>[3x]MAFSARFPLWLLLGVVLLASVSASFAHSGHSGGEAEDESEESRAQNNPYLFRSNKFLTLFKNQHGSLRLLQRFNEDTEKLENLRDYRVLEYCSKPNTLLLPHHSDSDLLVLVLEGQAILVLVNPDGRDTYKLDQGDAIKIQAGTPFYLINPDNNQNLRILKFAITFRRPGTVEDFFLSSTKRLPSYLSAFSKNFLEASYDSP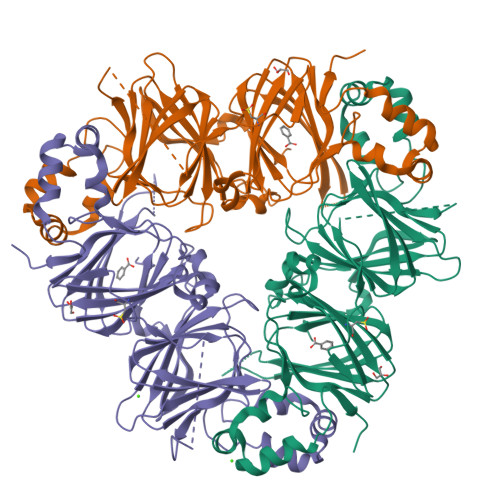YDEIEQTLLQEEQEGVIVKMPKDQIQEISKHAQSSSRKTLSSQDKPFNLRSRDPIYSNNYGKLYEITPEKNSQLRDLDILLNCLQMNEGALFVPHYNSRATVILVANEGRAEVELVGLEQQQQQGLESMQLRRYAATLSEGDIIVIPSSFPVALKAASDLNMVGIGVNAENNERNFLAGHKENVIRQIPRQVSDLTFPGSGEEVEELLENQKESYFVDGQPRHIDAGGKARRAHLPNLFRTFY> GAACGACACAGA;> CGTCGACTC;> TCTACG;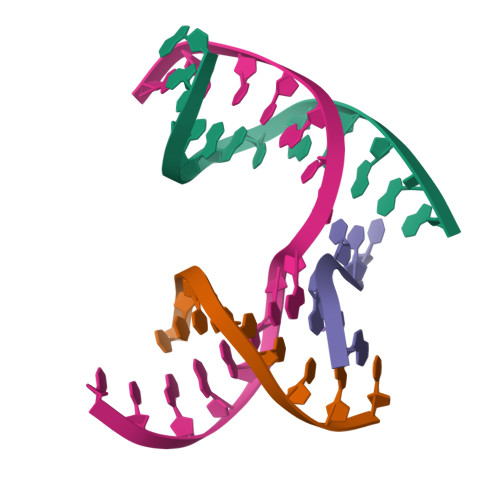> TCGAGTCGGTGTCGT>SLQRVPSYDSFDSEDYPAALPNHKPKGTFKDYVRDRADLNKDKPVIPAAALAGYTGSGPIQLWQFLLELLTDKSCQSFISWTGDGWEFKLSDPDEVARRWGKRKNKPKMNYEKLSRGLRYYYDKNIIHKTAGKRYVYRFVCDLQSLLGYTPEELHAMLDVKPDAD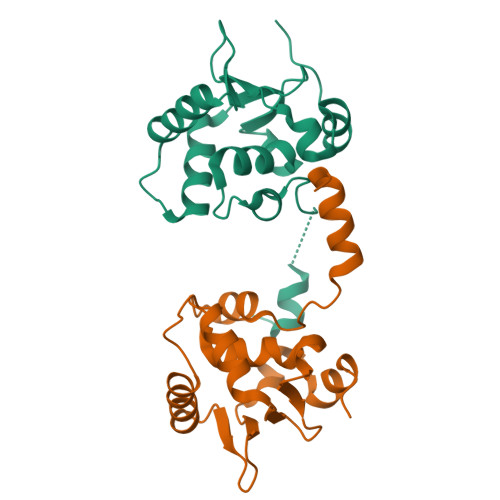E[2x]>MGSSHHHHHHSSGRENLYFQGMPRWLIQHSPNTLTPEEKSHLAQQITQAYVGFGLPAFYVQVHFIEQPAGTSFIGGEQHPNFVALTIYHLARTMTSDEQRQGFLKRIDAFLTPMFEPKG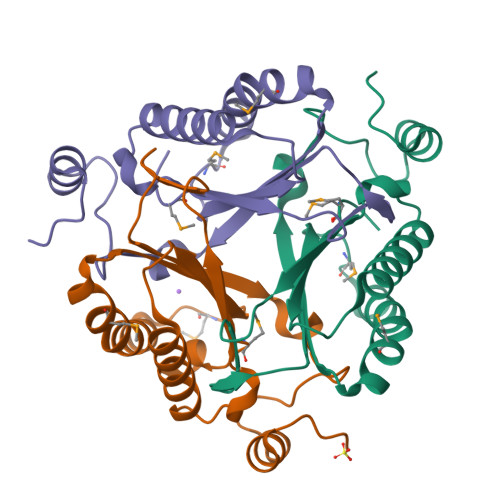IDWEYFVTEAPRDLWKINGLAPPAAGSEEEKVWVRENRPVRF[3x]The FfIBP from Flavobacterium frigoris PS1 exhibits high TH activity and relatively strong recrystallization inhibition activity. The FfIBP structure is composed of parallel β-strands in a helical pattern, which is mainly stabilized by inner hydrophobic interactions and intramolecular hydrogen bonds with long α415. Additionally, the FfIBP has a capping head region that consists of two small turns and β-strands, which contain a disulfide bond. This disulfide bond increases the overall rigidity of the protein and reduces residual movement at the ice-binding site, thereby augmenting TH activity and protein stability.

Based on the CD and MD simulation data, four mutants annotated as FfIBP_CC1 (A101C-A120C), FfIBP_CC2 (S96C-L132C), FfIBP_CC3 (M249C-N270C), and FfIBP_CC4 (G160C-S176C), possibly forming disulfide bonds, were generated. The FfIBP_CC2 is located at the interface between the body domain and the long α-helix (α4). To confirm the disulfide formation, we solved the crystal structures of the FfIBP_CC1, CC2, CC3, and CC4 at 2.0, 2.1, 2.0, and 2.0 Å, respectively. Successful formation of the disulfide bond at the intended location in FfIBP_CC1 and FfIBP_CC4 was confirmed by X-ray crystallography, whereas the rest did not form a disulfide bond. The failure to form a disulfide bond may be due to dihedral angle constraints and the inappropriate distance between the two cysteines. When the RMSD values of alpha carbon mutants were compared with the wildtype, relatively high RMSD values exceeding 0.4 Å were observed around the mutation sites of FfIBP_CC2, FfIBP_CC3, and FfIBP_CC4. In contrast, FfIBP_CC2 exhibited a drastic decrease in the melting temperature by approximately 8.3 °C. The mutation at the Ser96 and Lue132 to cysteines likely distorted the conformation of the residual interactions between the β helical body region and α4, which was vulnerable during thermal melting.

> HMSLSVANSTYETTALNSQKSSTDQPNSGSKSGQTLDLVNLGVAANFAILSKTGITDVYKSAITGDVGACPITGAAILLKCDEVTGTIFSVDAAGPACKITDASRCTTAVGDMQIAYDNAAGRLNPDFLNLGAGTIGGKTLTPGLYKWTSTLNIPTDITISGSSTDVWIFQVAGNLNMSSAVRITLAGGAQAKNIFWQTAGAVTLGSTSHFEGNILSQTGINMKTAASINGRMMAQTAVTLQMNTVTIPQ Doripenem 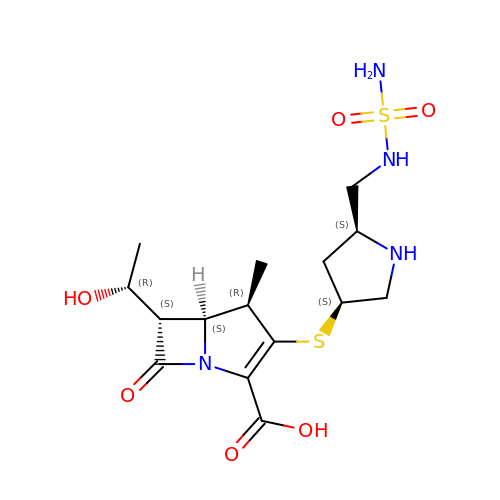| C15 H24 N4 O6 S2 | AVAACINZEOAHHE-VFZPANTDSA-N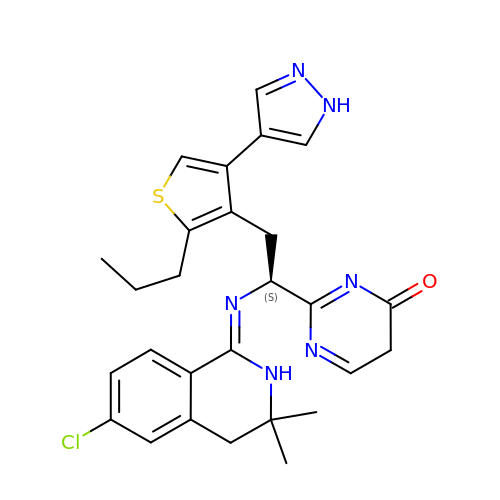2-{(1S)-1-{[(1Z)-6-chloro-3,3-dimethyl-3,4-dihydroisoquinolin-1(2H)-ylidene]amino}-2-[2-propyl-4-(1H-pyrazol-4-yl)thiophen-3-yl]ethyl}pyrimidin-4(5H)-one | C27 H29 Cl N6 O S | SHQGADSMADPNBQ-QFIPXVFZSA-N1-BROMOBUTANE | C4 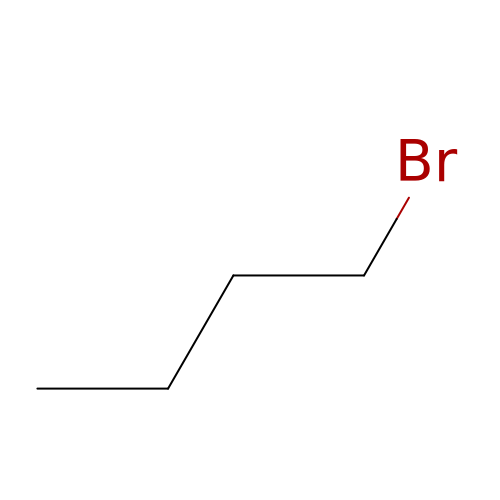H9 Br | MPPPKRYCTPRNTB-UHFFFAOYSA-N(2~{S})-2-azanyl-4-[4-[bis(4-fluorophenyl)methyl]piperazin-1-yl]-1-(1,3-dihydroisoindol-2-yl)butane-1,4-dione 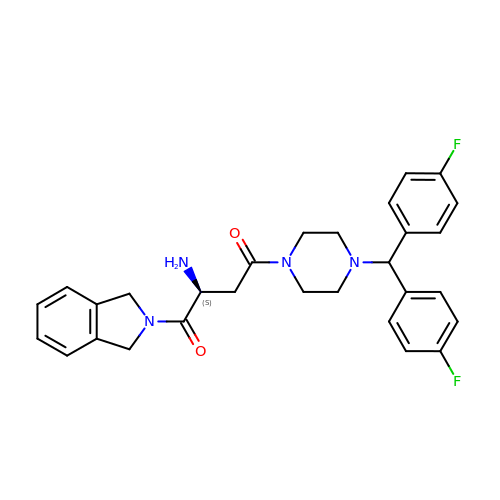| C29 H30 F2 N4 O2 | ZKIQFLSGMMYCGS-SANMLTNESA-N>MPYHEFEVSKCIPERREHAVMKAAGEDLTSCLPKGYLNTIPGTISERGCAYCGAKHVIGTPMKDVIHISHGPNGCTYDTWQTKRYISDNDNFQLKYTFATDVKEKHVVFGAEGLLKKSMHEAFDAFPNIKRMTVYQTCTTALIGDDVDAIAKEVMEERGDVDVFVCNSPGFAGPSQSGGHHKINIAWLNQKVGTVEPDYLGEHVINYVGEYNIQGDQEVMIDYFNRMGIQVLSTFTGNGSYDSLRMMHRAHLNVLECARSAEYICDELRARYGIPRLDIDGFGFEPLANSLRKVALFFGIEDKAEAIIAEEYAKWKPQLDWYKERLKGKKVCLWPGGSKLWHWAHAIEEEMGLKVVSVYTKFGHQGDMEKGVSRCGEGALAIDDPNELESVEAIEMLKPDIIFTGKRPGEFVKKHGVPYLNAHAYHNGPYKGFEGWVRFARDIYNAIYSPMRQLAALDISAPDAAITSGFRTAKMNADLTVSDEVKFSEVLHEYTGKYDSIAEIRARNQAYAAEQKALRDAVQPAAEWSHPQFEK[2x];>MTDISEKLDPLVDYIMKNCLWQFNSRGWDRLKQNAGILSQTCEILCGEEPVHETAMDRCYWVDAVILSRAYKARFPWLMAMTKPEIKSLFKALHEKIDHLTVHGSLNTELTVPHY[2x];>MTCQVTQKAREGTINPIFTCQPAGAQFASIGIKDCIGIVHGGQGCVMFVRLLISQHMKESFEIASSSVHEDGAVFGALDRVETAVEVLLTRYPDVKVVPIITTCSTEIIGDDVDGLLSKLEDELLPTKFPGREVHLLTVHCPSFVGSMITGYDKAVHDFVKKFATKDEPSDKINLITGWVNPGDVKELKHLLEVMEVKANVLFEVESFDSPLMPDLEHHSHGSTTIEDLRDTANAKGTIALNRYEGMKAADYLKKKFKVPAVIGPTPVGIRNTDAFLKAVSEMTGQPIPAQLVKERGLALDAIADIGHMFLADKRVAIYANPDLAIGLTEFCLDLEMKPKLLLLGDDNSGYVKDPRVLALQENAPDLEIVTNADFWDLESRIQQGLELDLILGHSKGRFISIDYKVPMVRVGFPTYDRAGMYRHPVLGYGGAMFLAETMANTLFADMEAKKNKEWILNVW[2x];>MTRKIAIYGKGGIGKSTTTQNTAAALAFFHEKNVFIHGCDPKADSTRLILGGLPQQTVMDTLRIEGAERVTVDKVVKTGFKDIRCVESGGPEPGVGCAGRGVITAIDLMEENEAYSEDLDFLFFDVLGDVVCGGFAMPIRDGKAEEVYIVASGEMMAIYAANNICKGLAKYARQSGVRLGGIICNSRNVDGEKEFLEEFTKAIGTKMIHFVPRDNIVQKAEFNKQTVTEFQPEANQAQEYRELGRKIIENEDFVIPKPLAMDELEAMVVKYGLMD[4x]

Nitrogenases catalyze a key step in the global nitrogen cycle by reducing molecular nitrogen (dinitrogen, N2) to ammonia (NH3). Some diazotrophs encode ‘back-up’ or alternative nitrogenase genes: vnfHDGK for the vanadium (V) nitrogenase or anfHDGK for the iron (Fe) nitrogenase, expressed upon the depletion of Mo. Upon complex formation, low-potential electrons are transferred from the [Fe4S4] cluster of the reductase component via an [Fe8S7] relay (P-cluster) to the active site cofactor of the catalytic component. The active site cofactor is expected to follow the general composition of [MFe7S9C-(R)-homocitrate], where M is Mo, V or Fe, depending on the nitrogenase isoform.

Using anaerobic single-particle cryogenic electron microscopy (cryo-EM), we solved the structure of the adenosine diphosphate-aluminum fluoride (ADP·AlF3)-stabilized Fe nitrogenase complex consisting of two reductase components and one catalytic component at a resolution of 2.35 Å. Following anaerobic sample preparation including plunge freezing inside an anaerobic tent, we obtained a 2.35-Å resolution map visualizing the expected heterodecameric complex of two AnfH2 dimers bound to Anf(DGK)2. Indeed, our structure contains one ATP mimic MgADP·AlF3 per AnfH subunit, locking the Fe nitrogenase complex in the transition state. In the dimeric interface of the reductase component, we observed an [Fe4S4] cluster coordinated by Cys97 and Cys132 of the two interacting AnfH subunits. In our structure, the [Fe4S4] cluster is 17.7 Å apart from the P-cluster. The P-cluster is in the dithionite-reduced PN state forming a symmetric molecule, connected by a shared sulfide ion and bound by six cysteine residues of either the D or K subunit. During catalysis, the P-cluster donates electrons to the FeFeco at a distance of 19.4 Å. As previously proposed, the FeFeco is an [Fe8S9C-(R)-homocitrate] cluster that, in contrast to the Mo and V nitrogenases, contains no transition metal other than iron (based on ICP-OES). Intriguingly, the G subunit contributes directly to the binding of AnfH2 through hydrogen bonding between His114AnfG and Asn112AnfH as well as Thr111AnfG and Arg69AnfH. Indeed, B factors around the αIII domain are the highest within the catalytic core of the Fe nitrogenase, hinting at an inherently flexible character of the αIII domain that is stabilized by the interaction with AnfG.> MALDRPDRSGAVRVSAPARLSFTLISLDGSSLRRNGIAAMAVDRPGLTAEVREAADGIVAVTGTAEETARELAAALEALRKLWDGPAARVDVLEALPQHSGFGSKTSTLLAVGHAYGRLCGVEPDLRELARTLGRGRTSGASTGLSAYGGFLVDGGHVNPPDFAEAPQKYLRPSRFAQQVAPPKPVVRLDFPDWPVLVLLTHGRHLGGQEELEWFHSVAPIPAEESWRTSHLVFMGLAPAVLEQDFDAFCAAVNEITFTGHFKQ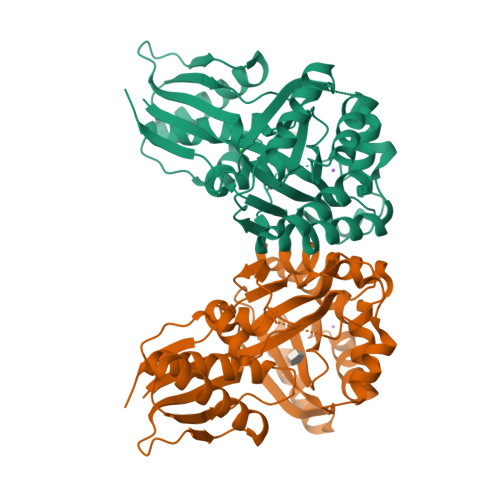AQIAFQGDAVADVLEAGRAAPSVDAIALSVTGPACFAFTKRPEDAERWAWELKNRGLIRDFWFTRANNQGLATTVVS> MRGSHHHHHHGSLDFAHPAYSAREQQWMADHPVVKVAVLNLFAPFTLFRTD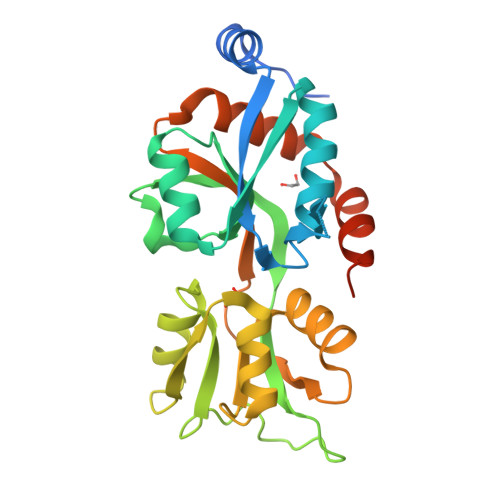EQFGGISAAVLQLLQLRTGLDFEIIGVDTVEELIAKLRSGEADMAGALEVNSARESFLSFSRPYVRNGMVIVTRQDPDAPVDADHLDGRTVALVRNSAAIPLLQRRYPQAKVVTADNPSEAMLMVANGQADAVVETQISASYYVNRYFAGKLRIASALDLPPAEIALATTRGQTELMSILNKALYSISNDELASIISRWRGSDGDPRTWYAYRNEI Dye-decolourising peroxidases (DyPs) are a distinct structural family of peroxidases possessing an α + β dimeric fold that houses a b-type heme coordinated on its proximal side by a His residue. The soil dwelling bacterium, Streptomyces lividans possesses three DyPs; two belonging to the A-type and a third belonging to the B-type sub-families. The two A-type homologs, named DtpA and DtpAa react in their ferric heme state with H2O2 to form a two-electron oxidised derivative that is an Fe(iv)O heme carrying a porphyrin π-cation radical (Fe(iv)O[Por˙+]) – termed compound I.34–36 In the presence of a substrate, reduction of the porphyrin π-cation radical results in the formation of compound II (Fe(iv)O), with a second substrate molecule reducing compound II to the ferric state. By using an A-type member of the DyP family (DtpAa) as an exemplar, we combine protein engineering, X-ray crystallography, hole-hopping calculations, EPR spectroscopy and kinetic modelling to provide compelling new insights into the control of radical migration pathways following reaction of the heme with hydrogen peroxide.

The Y345F variant, creates a DtpAa protein with no Tyr residues within 15 Å of the heme on the distal side with the double variant, Y345F/F347Y, mimicking the distal heme Tyr arrangement as in DtpA. High-resolution X-ray crystal structures determined to 1.23 Å (Y345F) and 1.27 Å (Y345F/F347) resolutions, corroborated the desired amino acid changes. The X-ray crystal structure of the double variant reveals that the Asp358 side chain undergoes a positional change, relative to that observed in the Y345F variant and WT DtpAa, enabling for a H-bond network to form with a newly appeared H2O molecule and the Tyr347 phenol group. This arrangement mimics the proton acceptor architecture identified in DtpA, considered important for creating a stable YO˙ species. Not surprisingly, the fastest hole hopping pathways (τM 10−3 s) in the Y345F and double variant remain dominated by the proximal Trp/Tyr dyad. However, in the double variant, a hole hopping pathway is calculated (P3), with a τM value on the same order of magnitude to that calculated for the Tyr374 pathway in DtpA. Thus, the introduction in DtpAa of a Tyr at position 347 distal to the heme facilitates a new hole hopping pathway. In the case of the double variant (mimics the Tyr arrangement of the distal heme in DtpA), a lowly populated EPR signal, with a maximal intensity at ∼3 min was detected. The line shape and position, albeit of a low signal-to-noise ratio, are consistent with a possibility of the signal being caused by a YO˙ species. In the double variant, although the engineered distal Tyr347 is present, and indeed identified as the YO˙ species in the triple variant, it is minimally populated.

>[2x]MTDTDSPAPAPSPSRRSLIGWGGAGLALGAAAAAGGAVAMDRAGADADPAGADAGSAVPFHGAHQAGIATPVQDRLHFAAFDVTTEDRAAFVALLKEWTAAARRLTAGHAVGEGAYGGLPEAPPDDTGEALGLKPSRLTLTIGFGPSLFTRFGLADLRPEALADLPKFPGDNLDRARSGGDLCVQACADDPQVAVHAIRNLARIGFGKVVVRWSQLGFGKTSSTTPDKQTPRNLLGFKDGTRNIAGTEKDRLDRFVWAAEKDGTPWMTGGSYLVARRIRMHIETWDRASLQEQEDVFGRDKGEGAPVGKAKERDEPFLKAMKPDAHVRLAHPDSNGGATLLRRGFSYTDGTDGLGRLDAGLFFLAYQRDIRTGFVPVQRNLATDALNEYIQHVGSAVFAVPPGVRDADDWWGSTLFG> VADRGQRRGCAPGIASALRASFQGKSRPWTQTRYWAFALLTPLVVAMVLTGCSASGTQLELAPTADRRAAVGTTSDINQQDPATLQDGGNLRLSLTDFPPNFNILHIDGNNAEVAAMMKATLPRAFIIGPDGSTTVDTNYFTSIELTRTAPQVVTYTINPEAVWSDGTPITWRDIASQIHAISGADKAFEIASSSGAERVASVTRGVDDRQAVVTFAKPYAEWRGMFAGNGMLLPASMTATPEAFNKGQLDGPGPSAGPFVVSALDRTAQRIVLTRNPRWWGARPRLDSITYLVLDDAARLPALQNNTIDATGVGTLDQLT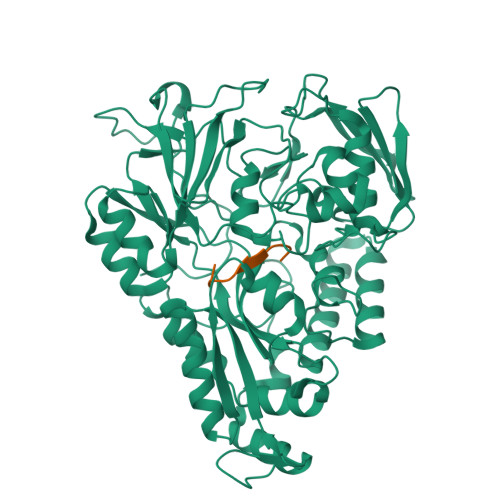IAARTKGISIRRAPGPSWYHFTLNGAPGSILADKALRLAIAKGIDRYTIARVAQYGLTSDPVPLNNHVFVAGQDGYQDNSGVVAYNPEQAKRELDALGWRRSGAFREKDGRQLVIRDLFYDAQSTRQFAQIAQHTLAQIGVKLELQAKSGSGFFSDYVNVGAFDIAQFGWVGDAFPLSSLTQIYASDGESNFGKIGSPQIDAAIERTLAELDPGKARALANQVDELIWAEGFSLPLTQSPGTVAVRSTLANFGATGLADLDYTAIGFMRRHHHHHHHH;> ASPFSPDPP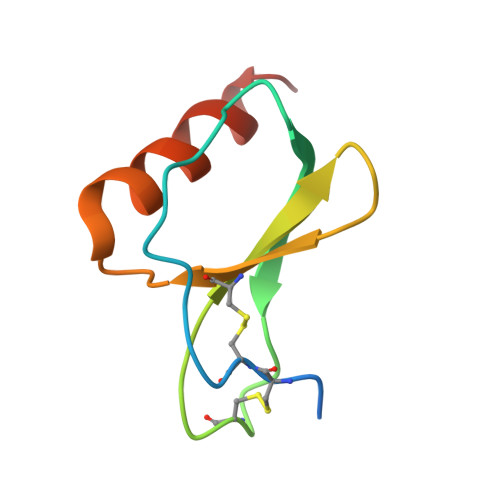>[2x]ARGTNVGRECCLEYFKGAIPLRKLKTWYQTSEDCSRDAIVFVTVQGRAICSDPNNKRVKNAVKYLQSLERS>[6x]MRLSYEALEWRTPIENSTEPVSLPPPPPFFGQERAREALELAIRGGFHAYLVGPPSLGKHEALLAYLSTQSVETPPDLLYVPLSERKVAVLTLPSGQEIHLAEAVEGLLLEVNRLDELFRQGSFLREKTQLEARFKEAREQQLEALRREAQEAGFALSTNGERLELTGPGPVPAELSARLEEVTLGSLAASAELEVALRRLRRDWALHYLNNRFEPLFQRFPQARAYLEALRARLARYAETGEPLDPAQWRPNLLTSSSSGTPPPIVYEPYATAPRLFGRLDYLVDRGVWSTNVSLIRPGAVHRAQGGYLILDALSLKREGTWEAFKRALRNGQVEPVTEPQAPAGLEVEPFPIQMQVILVGTPEAFEGLEEDPAFSELFRIRAEFSPTLPASPENCTALGGWLLAQGFQLTQGGLTRLYDEARRMAEQRDRMDARLVEIRALAEEAAVLGGGLLTAESVEQAIAAREHRSF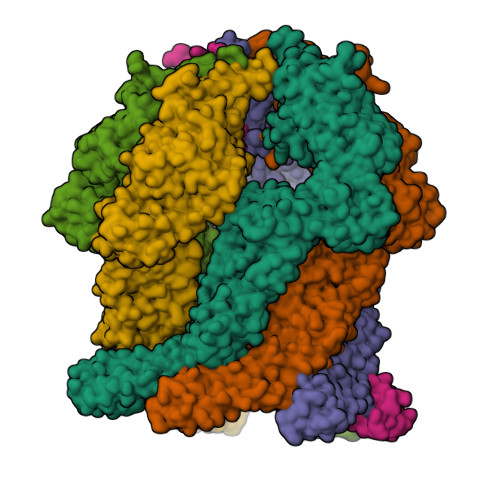LSEEEFLRAVQEGVIRLRTTGRAVGEVNSLVVVEAAPYWGRPARLTARAAPGRDHLISIDREAGLGGQIFHKAVLTLAGYLRSRYIEHGSLPVTISLAFEQNYVSIEGDAAGLAELVAALSAIGNLPLRQDLAVTGAVDQTGKVLAVGAINAKVEGFFRVCKALGLSGTQGVILPEANLANLTLRAEVLEAVRAGQFHIYAVETAEQALEILAGARMEGFRGLQEKIRAGLEAFARLEEGHDKEDREKLAAALEHHHHHH>[2x]SNPNRILP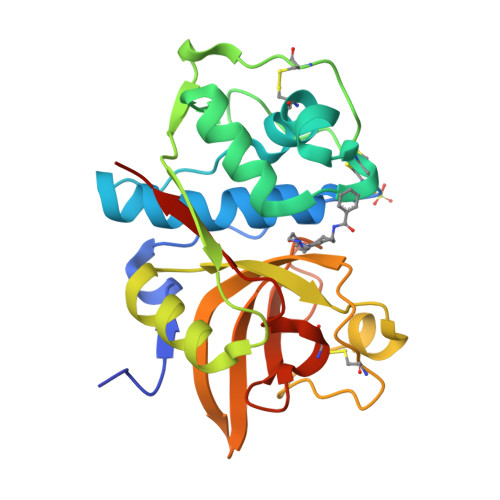DSVDWREKGCVTEVKYQGSCGACWAFSAVGALEAQLKLKTGKLVSLSAQNLVDCSTEKYGNKGCNGGFMTTAFQYIIDNKGIDSDASYPYKAMDQKCQYDSKYRAATCSKYTELPYGREDVLKEAVANKGPVSVGVDARHPSFFLYRSGVYYEPSCTQNVNHGVLVVGYGDLNGKEYWLVKNSWGHNFGEEGYIRMARNKGNHCGIASFPSYPEIEHHHHHH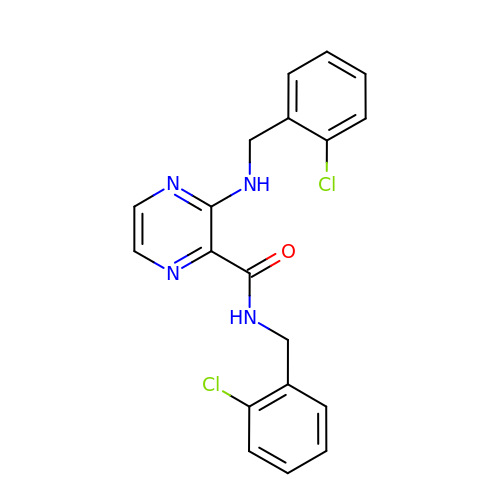~{N}-[(2-chlorophenyl)methyl]-3-[(2-chlorophenyl)methylamino]pyrazine-2-carboxamide | C19 H16 Cl2 N4 O | ODVHBUXWRYPLHQ-UHFFFAOYSA-N>LQHHHHHHHHASQNDTEPIVLEGKCLVVCDSNPATDSKGSSSSPLGISVRAANSKVAFSAVRSTNHEPSEMSNKTRIIYFDQILVNVGNFFTLESVFVAPRKGIYSFSFHVIKVYQSQTIQVNLMLNGKPVISAFAGD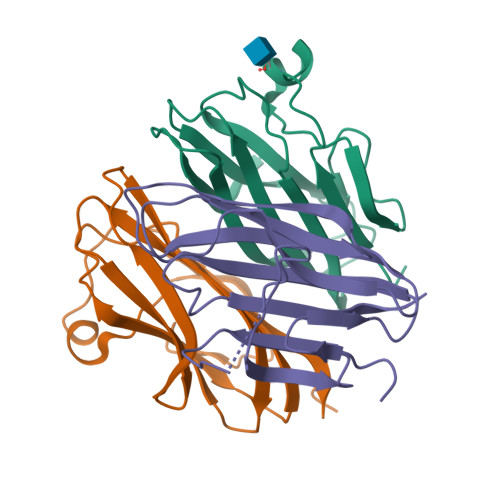KDVTREAATNGVLLYLDKEDKVYLKLEKGNLLGGWQYSTFSGFLVFPL[3x]N-NAPHTHALEN-1-YLMETHYL-2'-[3,5-DIMETHOXYBENZAMIDO]-2'-DEOXY-ADENOSINE 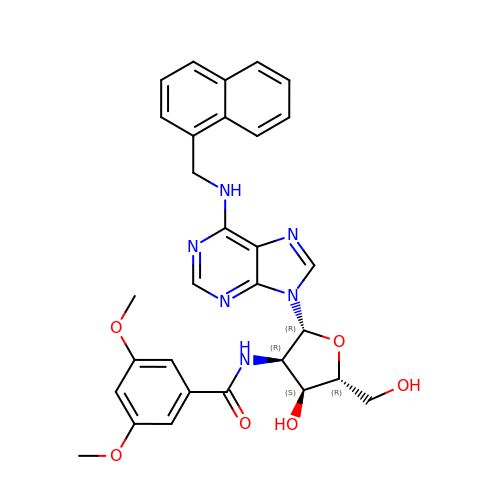| C30 H30 N6 O6 | OARVXDFNTLYMCJ-JVUUKAHWSA-N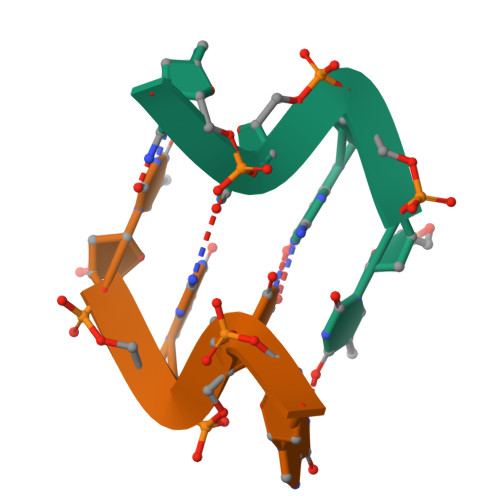>TGTG[2x]6-(2-(5-(3-(DIMETHYLAMINO)PROPYL)PYRIDIN-3-YL)ETHYL)-4-METHYLPYRIDIN-2-AMINE 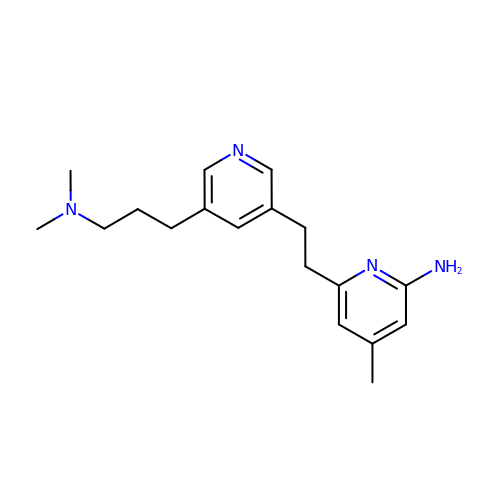| C18 H26 N4 | TUAXAWZDVAYXFN-UHFFFAOYSA-N> DPAGLLDLRQGMFAQLVAQNVLLIDGPLSWYSDPGLAGVSLTGGLSYKEDTKELVVAKAGVYYVFFQLELRRV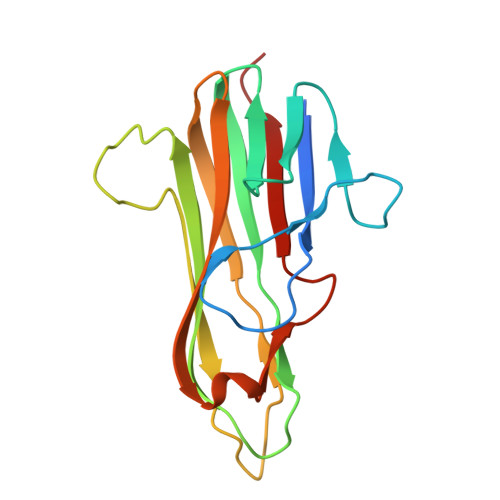VAGEGSGSVSLALHLQPLRSAAGAAALALTVDLPPASSEARNSAFGFQGRLLHLSAGQRLGVHLHTEARARHAWQLTQGATVLGLFRVTPEI> GPHMLEMVTDQFGMIGLLTFIRAAETDPGMVHLALGSDLTTLGLNLNSPENLYPKFASPWASSPCRPQDIDFHVPSEYLTNIHIRDKLAAIKLGRYGEDLLFYLYYM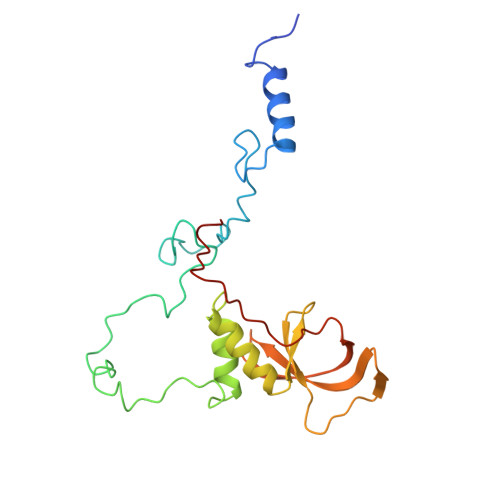NGGDVLQLLAAVELFNRDWRYHKEERVWITRAPGMEPTMKTNTYERGTYYFFDCLNWRKVAKEFHLEYDKLEERPHLPSTFNYNPAQQAF>[2x]MKNNKIYLLGACLLCAVTTFAQNVSLQPPPQQLIVQNKTIDLPAVYQLNGGEEANPHAVKVLKELLSGKQSSKKGMLISIGEKGDKSVRKYSRQIPDHKEGYYLSVNEKEIVLAGNDERGTYYALQTFAQLLKDGKLPEVEIKDYPSVRYRGVVEGFYGTPWSHQARLSQLKFYGKNKMNTYIYGPKDDPYHSAPNWRLPYPDKEAAQLQELVAVANENEVDFVWAIHPGQDIKWNKEDRDLLLAKFEKMYQLGVRSFAVFFDNISGEGTNPQKQAELLNYIDEKFAQVKPDINQLVMCPTEYNKSWSNPNGNYLTTLGDKLNPSIQIMWTGDRVISDITRDGISWINERIKRPAYIWWNFPVSDYVRDHLLLGPVYGNDTTIAKEMSGFVTNPMEHAESSKIAIYSVASYAWNPAKYDTWQTWKDAIRTILPSAAEELECFAM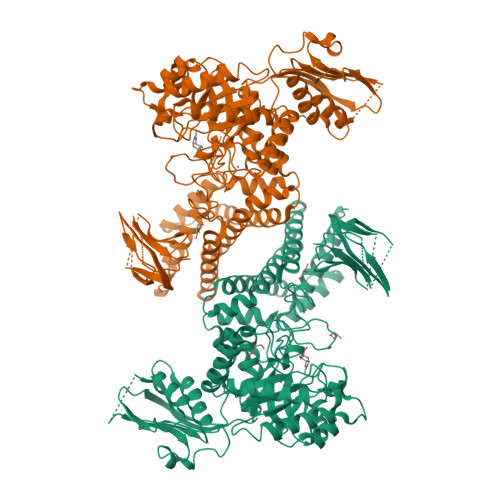HNSDLGPNGHGYRREESMDIQPAAERFLKAFKEGKNYDKADFETLQYTFERMKESADILLMNTENKPLIVEITPWVHQFKLTAEMGEEVLKMVEGRNESYFLRKYNHVKALQQQMFYIDQTSNQNPYQPGVKTATRVIKPLIDRTFATVVKFFNQKFNAHLDATTDYMPHKMISNVEQIKNLPLQVKANRVLISPANEVVKWAAGNSVEIELDAIYPGENIQINFGKDAPCTWGRLEISTDGKEWKTVDLKQKESRLSAGLQKAPVKFVRFTNVSDEEQQVYLRQFVLTIEKK> VVGGTDADEGEWPWQVSLHALGQGHICGASLISPNWLVSAAHCYIDDRGFRYSDPTQWTAFLGLHDQSQ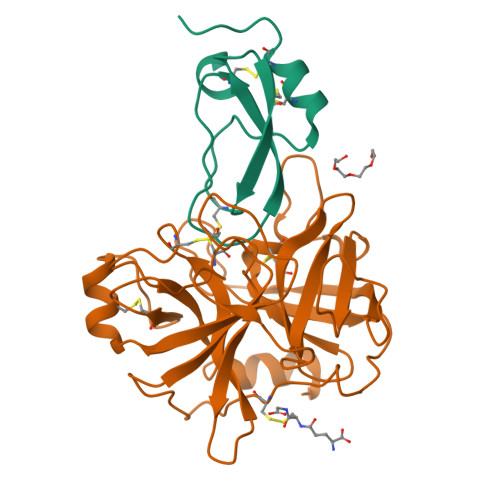RSAPGVQERRLKRIISHPFFNDFTFDYDIALLELEKPAEYSSMVRPICLPDASHVFPAGKAIWVTGWGHTQYGGTGALILQKGEIRVIQQTTCENLLPQQITPRMMCVGFLSGGVDSCQGDSGGPLSSVEADGRIFQAGVVSWGDGCAQRNKPGVYTRLPLFRDWIKENTGV;> QTEDYCLASNKVGRCRGSFPRWYYDPTEQICKSFVYGGCLGNKNNYLREEECILACRGVQGP Mimivirus is the prototype of the Mimiviridae family of giant dsDNA viruses. Little is known about the organization of the 1.2 Mb genome inside the membrane-limited nucleoid filling the ~0.5 µm icosahedral capsids. Cryo-electron microscopy, cryo-electron tomography, and proteomics revealed that it is encased into a ~30-nm diameter helical protein shell surprisingly composed of two GMC-type oxidoreductases, which also form the glycosylated fibrils decorating the capsid. The genome is arranged in 5- or 6-start left-handed super-helices, with each DNA-strand lining the central channel.

In the relaxed subcluster Cl3a, the DNA strands at the interface to the ~17-nm-wide central channel are not clearly recognizable, most likely because they are at least partially detached inside the broken expanded fiber. The breaks after relaxation of the helix might be the result of the extraction and purification treatment, while DNA will remain in the central channel, at least in the early phase of Acanthamoeba infection. The transition from Cl1a to Cl3a (5-start helix) corresponds to a rotation of each individual unit (corresponding to a GMC-oxidoreductase dimer) by ~−10° relative to the fiber longitudinal axis and a change in the steepness of the helical rise by ~−11°. The N-terminal chain, being more disordered than the rest of the structure, it is absent in the focused refined map, and also absent in the Cl3a map of the relaxed helix, suggesting that a break of the disulfide bridge could be involved in the observed unwinding process. Density that can be attributed to the FAD cofactor is also present in the Cl2 and Cl3a maps. The atomic models of Cl1a and Cl3a dimers are superimposable with a core root-mean-square deviation (RMSD) of 0.68 Å based on Cα atoms.

> MAHRSRCNCNDTSNSNGSQHGINLPLRKIDTYDPCVNCRVKPHLCPKPHPCPKPENLEADIVIIGAGAAGCVLAYYLTKFSDLKIILLEAGHTHFNDPVVTDPMGFFGKYNPPNENIRMSQNPSYAWQPALEPDTGAYSMRNVVAHGLAVGGSTAINQLNYIVGGRTVFDNDWPTGWKYDDIKKYFRRVLADISPIRDGTKVNLTNTILESMRVLADQQVSSGVPVDFLINKATGGLPNIEQTYQGAPIVNLNDYEGINSVCGFKSYYVGVNQLSDGSYIRKYAGNTYLNSYYVDSNGFGIGKFSNLRVISDAVVDRIHFEGQRAVSVTYIDKKGNLHSVKVHKEVEICSGSFFTPTILQRSGIGDFSYLSSIGVPDLVYNNPLVGQGLRNHYSPITQVSVTGPDAAAFLSNTAAGPTNMSFRGAGMLGYHKLEPNKPSNAGSVTYRKYELLVTGGVAISADQQYLSGISSSTGNYFALIADDIRFAPVGYIKIGTPNFPRDTPKIFFNTFVNYTPTTDPADQQWPVAQKTLAPLISALLGYDAIYQIVQQMKVVAVNAGFNVTLQMAYPPNDLLVELHNGLNTYGINWWHYFVPSLVNDDTPAGKLFASTLSKLSYYPRSGAHLDSHQSCSCSIGGTVDTELKVIGVENVRVTDLSAAPHPPGGNTWCTAAMIGARATDLILGKPLVANLPPEDVPVFTTS> GSRISAEGSQACAKGCELCSEVNGC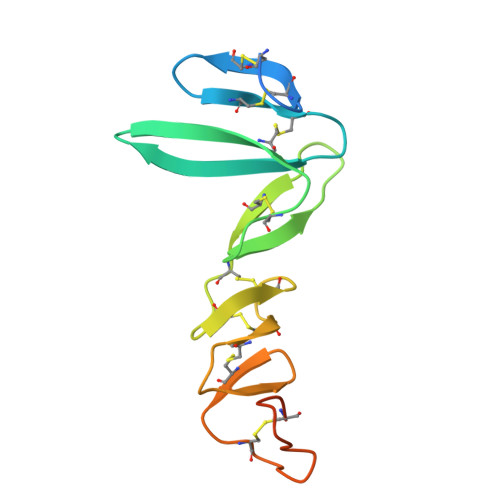LKCSPKLFILLERNDIRQVGVCLPSCPPGYFDARNPDMNKCIKCKIEHCEACFSHNFCTKCKEGLYLHKGRCYPACPEGSSAANGTMECSSPAAAHHHHHH> MFTFIKKVIKTGTATSSYPLEPIAVDKNFRGKPEQNPQQCIGCAACVNACPSNALTVETDLATGELAWEFNLGHCIFCGRCEEVCPTAAIKLSQEYELAVWKKEDFLQQSRFALCNCRVCNRP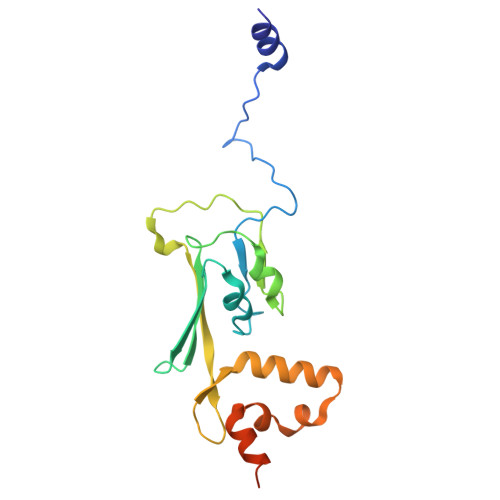FAVQKEIDYAIALLKHNGDSRAENHRESFETCPECKRQKCLVPSDRIELTRHMKEAI>MSLSNYIAGTLSFYVLRNPDLDRELINDYAPYSSSISIFEYHIAPNGDIANQLNDAAAIETTWQRRVTPLATITNLTSGG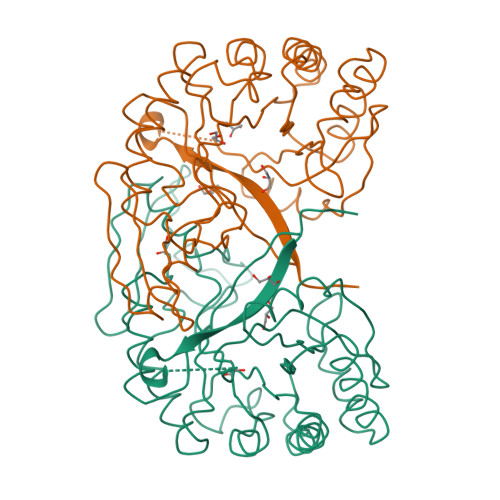FSTEIVHQVLNNPTARTNLVNNIYDLVSTRGYGGVTIDFEQVSAADRDLFTGFLRQLRDRLQAGGYVLTIAVPAKTSDNIPWLRGYDYGGIGAVVNYMFIMAYDWHHAGSEPGPVAPITEIRRTIEFTIAQVPSRKIIIGVPLYGYDWIIPYQPGTVASAISNQNAIERAMRYQAPIQYSAEYQSPFFRYSDQQGRTHEVWFEGVRSMSRKMQIVREYRLQAIGAWQLTLAEGHHHHHH[2x]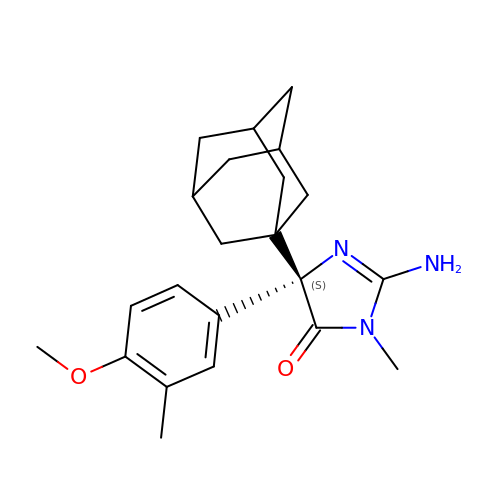(5S)-2-amino-5-(4-methoxy-3-methylphenyl)-3-methyl-5-[(3S,5S,7S)-tricyclo[3.3.1.1~3,7~]dec-1-yl]-3,5-dihydro-4H-imidazol-4-one | C22 H29 N3 O2 | HZIOSWLCMNAEBB-HJBSZYCQSA-N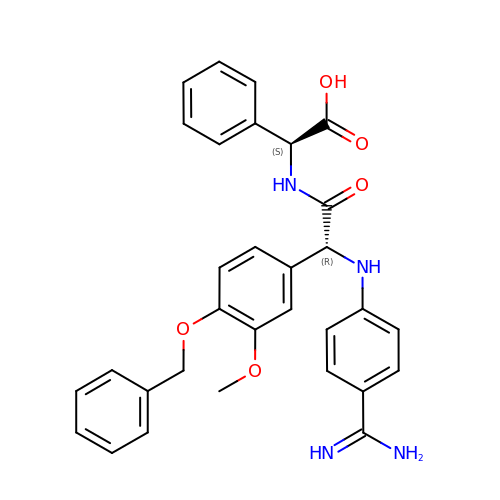(S)-[(R)-2-(4-BENZYLOXY-3-METHOXY-PHENYL)-2-(4-CARBAMIMIDOYL-PHENYLAMINO)-ACETYLAMINO]-PHENYL-ACETIC ACID | C31 H30 N4 O5 | WGEGXJPYFSZDMU-IZLXSDGUSA-N> HKCDITLQEIIKTLNSLTEQKTLCTELTVTDIFAASKNTTEKETFCRAATVLRQFYSHHEKDTRCLGATAQQFHRHKQLIRFLKALDRNLWGLAGLNSCPVKEANQSTLENFLERLKTIMREKYSKCSS

Interleukin 4 (IL-4) is a pleiotropic cytokine that plays a major regulatory role in the immune system. Signal transduction of IL-4 is mediated by a sequential binding process, initiated first by binding of IL-4 to its high-affinity single membrane spanning receptor chain IL-4Rα. This intermediate ligand receptor complex then recruits one of two possible low-affinity receptor subunits, the common gamma chain (γc) or the IL-13Rα1 chain, into the functional hetero-trimeric complex to initiate signalling. The overall structure of IL-4 comprises the known four-helical bundle in up-up-down-down topology, which like the crystal packing is unaffected by these mutations.

We tested the interaction model proposed above by mutating Arg85 of IL-4 and the super-agonistic variants to alanine and measuring the residual binding affinity to IL-4Rα. Changing Arg85 of IL-4 to alanine does not change the binding affinity for IL-4Rα dramatically (KD (R85A)/KD (wt IL-4) ~ 4.7-fold, thus ΔΔG = 1 kcal mol-1). This is in line with the observation that residues in Cluster III do not generally contribute to the overall binding. In particular, the dissociation rate constant is only increased by a factor less than 1.3, showing that the hydrogen-bonding network of Arg85 with IL-4Rα provides no free binding energy. To exclude the possibility that structural changes in addition to the removal of the Arg85 side chain play a role in the changes in binding stability, we determined the structures of the IL-4 variants R85A, T13D-R85A and F82D-R85A. No changes in the local structure around residues Thr/Asp13, Phe/Asp82 or Arg85 could be observed (data not shown).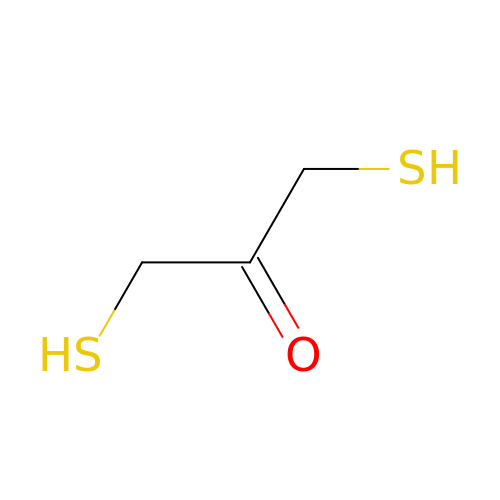1,3-bis(sulfanyl)propan-2-one | C3 H6 O S2 | QCBZCEKWIGTIMT-UHFFFAOYSA-N> SGLRGTFGGNIIQHSIPAVELRQPFFPTHMGPIKLRQFHRPPLKKYSFGALSQPGPHSVQPLLKHIKKKAKMREQERQASGGGEMFFMRTPQDLTGKDGDLILAEYSEENGPLMMQVGMATKIKNYYKRKPGKDPGAPDCKYGETVYCHTSPFLGSLHPGQLLQAFENNLFRAPIYLHKMPETDFLIIRTRQGYYIRELVDIFVVGQQCPLFEVPGPNSKRANTHIRDFLQVFIYRLFWKSKDRPRRIRMEDIKKAFPSH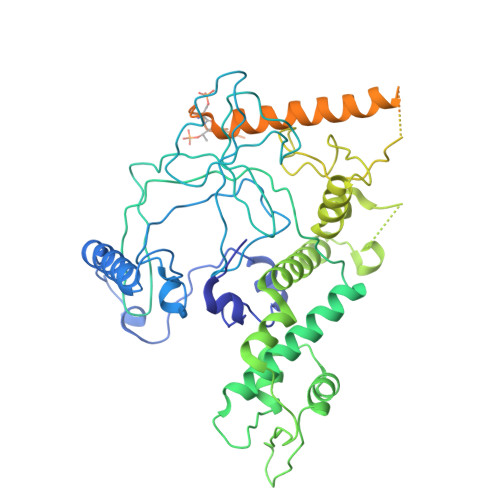SESSIRKRLKLCADFKRTGMDSNWWVLKSDFRLPTEEEIRAMVSPEQCCAYYSMIAAEQRLKDAGYGEKSFFAPEEENEEDFQMKIDDEVRTAPWNTTRAFIAAMKGKCLLEVTGVADPTGCGEGFSYVKIPNKPTQQKDDKEPQPVKKTVTGTDADLRRLSLKNAKQLLRKFGVPEEEIKKLSRWEVIDVVRTMSTEQARSGEGPMSKFARGSRFSVAEHQERYKEECQRIFDLQNKVLSSTEVLSTDTDSSSAEDSDFEEMGKNIENMLQNKKTSSQLSREREEQERKELQRMLLAAGSAASGNNHRDDDTASVTSLNSSATGRCLKIYRTFRDEEGKEYVRCETVRKPAVIDAYVRIRTTKDEEFIRKFALFDEQ>[2x]UAAGGAGGUGAU;>AUCACCUCCU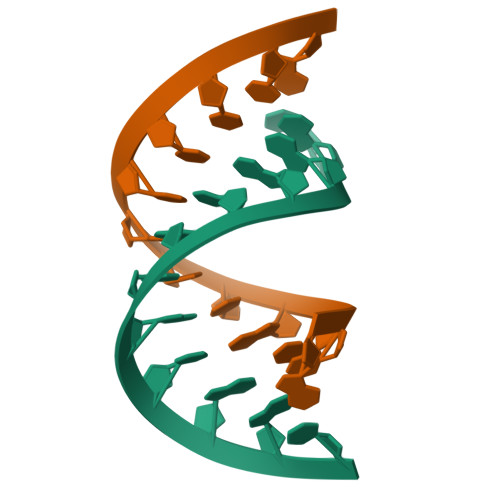UA[2x]>MKRDGHTHTEFCPHGTHDDVEEMVLKAIELDFDEYSIVEHAPLSSEFMKNTAGDKEAVTTASMAMSDLPYYFKKMNHIKKKYASDLLIHIGFEVDYLIGYEDFTRDFLNEYGPQTDDGVLSLHFLEGQGGFRSIDFSAEDYNEGIVQFYGGFEQAQLAYLEGVKQSIEADLGLFKPRRMGHISLCQKFQQFFGEDTSDFSEEVMEKFRVILALVKKRDYELDFNTAGLFKPLCGETYPPKKIVTLASELQIPFVYGSDSHGVQDIGR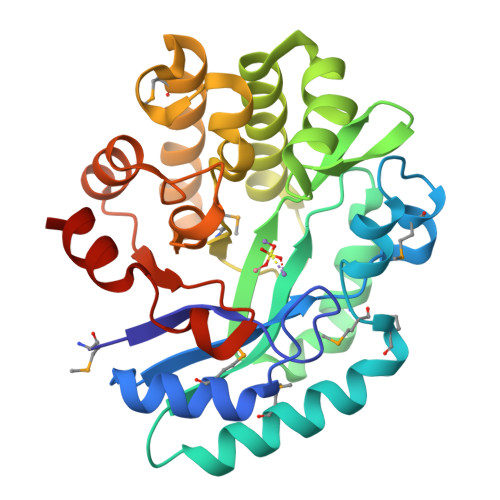GYSTYCQKLEHHHHHH[3x]>[2x]GSAMDVRQSIHSAHAKTLDTQGLRNEFLVEKVFVADEY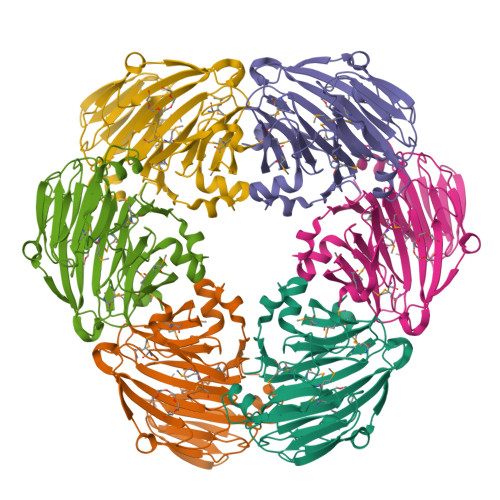TMVYSHIDRIIVGGIMPITKTVSVGGEVGKQLGVSYFLERRELGVINIGGAGTITVDGQCYEIGHRDALYVGKGAKEVVFASIDTGTPAKFYYNCAPAHTTYPTKKVTPDEVSPVTLGDNLTSNRRTINKYFVPDVLETCQLSMGLTELAPGNLWNTMPCHTHERRMEVYFYFNMDDDACVFHMMGQPQETRHIVMHNEQAVISPSWSIHSGVGTKAYTFIWGMVGENQVFDDMDHVAVKEICA Siroheme is the modified isobacteriochlorin tetrapyrrole used by siroheme-dependent sulfite and nitrite reductases (SiR/NiRs) in catalyzing the six-electron reduction of sulfite to sulfide or nitrite to ammonia. CysG is encoded by a gene fusion between a C-terminal SUMT (CysGA) and an N-terminal bifunctional dehydrogenase/ferrochelatase (CysGB). The N-terminal enzyme module, CysGB, is a three-domain bifunctional dehydrogenase/ATP-independent class III ferrochelatase12 that performs the final two steps of siroheme biosynthesis. The C-terminal enzyme module, CysGA, is homologous to a well-studied class of SAM-dependent uro’gen III methyltransferases (SUMTs) that catalyzes the methylations to generate precorrin-210,13.

D104 has been implicated in its chelatase activity but its exact role is unknown. Alteration to alanine results in an enzyme that cannot complement the cysG deficiency and is inactive for both dehydrogenase and chelatase activities. The D104A and D104N structures were determined to ensure that there were no gross structural defects that arose from the alterations that might impact their function. Indeed, both altered enzymes were crystallized and the structures are largely similar to Met8p. In the D104A structure, there is a slight movement of the DAPK loop in the closed, but not open, active site, highlighting the asymmetry of the active sites. In CysG, the D104A variant is catalytically inactive for both activities, supporting the idea that the side chain serves as a general base to facilitate proton abstraction in both reactions. D104A CysG is deficient in both dehydrogenase and ferrochelatase activities, whereas D104N activity is only partially reduced. Both D104 variants show buildup of a fluorescent intermediate, owing to the active SUMT.

>MDHLPIFCQLRDRDCLIVGGGDVAERKARLLLEAGARLTVNALTFIPQFTVWANEGMLTLVEGPFDETLLDSCWLAIAATDDDTVNQRVSDAAESRRIFCNVVAAPKAASFIMPSIIDRSPLMVAVSAGGTSPVLARLLREKLESLLPQHLGQVARYAGQLRARVKKQFATMGERRRFWEKFFVNDRLAQSLANADEKAVNATTERLFSEPLDHRGEVVLVGAGPGDAGLLTLKGLQQIQQADIVVYDRLVSDDIMNLVRRDADRVFVGKRAGYHCVPQEEINQILLREAQKGKRVVRLKGGDPFIFGRGGEELETLCHAGIPFSVVPGITAASGCSAYSGIPLTHRDYAQSVRLVTGHLKTGGELDWENLAAEKQTLVFYMGLNQAATIQEKLIAFGMQADMPVALVENGTSVKQRVVHGVLTQLGELAQQVESPALIIVGRVVALRDKLNWFSNH[2x]>[2x]GGSMLTLIQGKKIVNHLRSRLAFEYNGQLIKILSKNIVAVGSLRREEKMLNDVDLLIIVPEKKLLKHVLPNIRIKGLSFSVKVCGERKCVLFIEWEKKTYQLDLFTALAE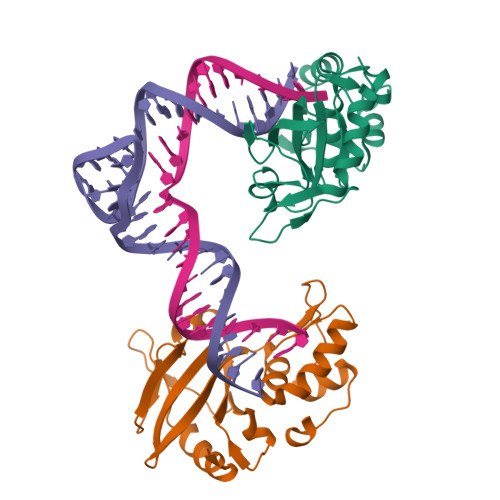EKPYAIFHFTGPVSYLIRIRAALKKKNYKLNQYGLFKNQTLVPLKITTEKELIKELGFTYRIPKKRL>[2x]SNAMPLTDTPPSVPQKPRRGRPRGAPDASL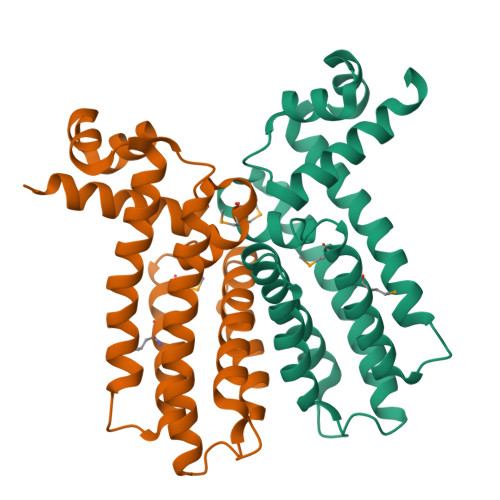AHQSLIRAGLEHLTEKGYSSVGVDEILKAARVPKGSFYHYFRNKADFGLALIEAYDTYFARLLDQAFLDGSLAPLARLRLFTRMAEEGMARHGFRRGCLVGNLGQEMGALPDDFRAALIGVLETWQRRTAQLFREAQACGELSADHDPDALAEAFWIGWEGAILRAKLELRPDPLHSFTRTFGRHFVTRTQE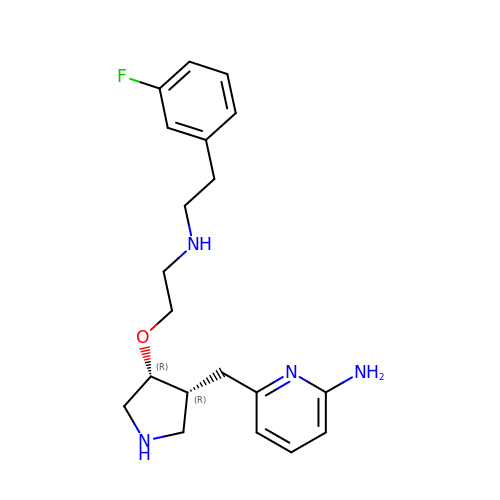6-{[(3R,4R)-4-(2-{[2-(3-fluorophenyl)ethyl]amino}ethoxy)pyrrolidin-3-yl]methyl}pyridin-2-amine | C20 H27 F N4 O | LRTPFJLYXDIXQR-APWZRJJASA-N2-oxidanyl-7-(pyrazol-1-ylmethyl)-3~{H}-1,4,2-benzodioxaborinine-8-carboxylic acid | C12 H11 B N2 O5 | 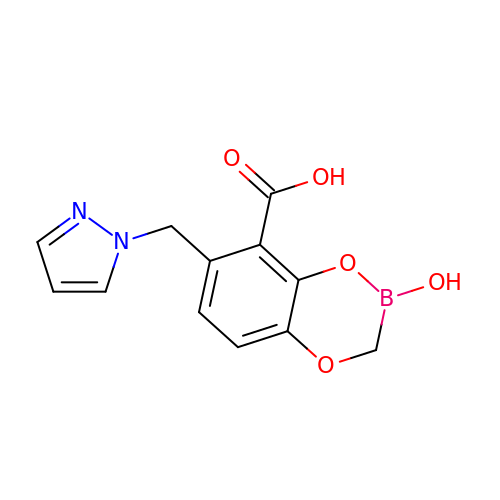VHKIDNUOLGPNSF-UHFFFAOYSA-N> GSHMRPLPAGLTASQQWTLLEWIHMAGHIETENELKAFLDQVLSQAPSERLLLALGRLNNQNQIQRLERVLNVSYPSDWLDQYMKENYAQHDPILRIHLGQGPVMWEERFNRAKGAEEKRFIAEATQNGMGSGITFSAASERNNIGSILSIAGREPGRNA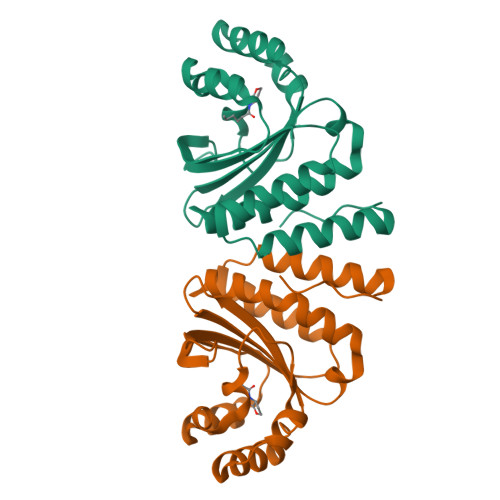ALVAMLNCLTPHLHQAAIRVAN>[4x]SKPFTVPILTVEEMTNSRFPIPLEKLFTGPSGAFVVQPQNGRCTTDGVLLGTTQLSPVNICTFRGDVTHIAGTHNYTMNLASQNWNNYDPTEEIPAPLGTPDFVGRIQGMLTQTTRGDGSTRGHKATVSTGDVHFTPKLGSIQFNTDTNNDFETGQNTKFTPVGVVQDGNGAHQNEPQQWVLPS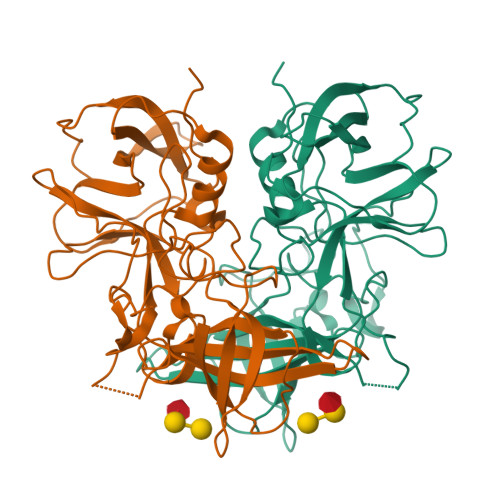YSGRTGHNVHLAPAVAPTFPGEQLLFFRSTMPGCSGYPNMNLDCLLPQEWVQHFYQEAAPAQSDVALLRFVNPDTGRVLFECKLHKSGYVTVAHTGQHDLVIPPNGYFRFDSWVNQFYTLAPM> GAGEMRDRIESMFLESWRDYSKHGWGYDVYGPIEHTSHNMPRGNQPLGWIIVDSVDTLMLMYNSSTLYKSEFEAEIQRSEHWINDVLDFDIDAEVNVFETTIRMLGGLLSAYHLSDVLEVGNKTVYLNKAIDLGDRLALAFLSTQTGIPYSSINLHSGQAVKNHADGGASSTAEFTTLQMEFKYLAYLTGNRTYWELVERVYEPLYKNNDLLNTYDGLVPIYTFPDTGKFGASTIRFGSRGDSFYEYLLKQYLLTHETLYYDLYRKSMEGMKKHLLAQSKPSSLWYIGEREQGLHGQLSPKMDHLVCFMGGLLASGSTEGLSIHEARRRPFFSKSDWDLAKG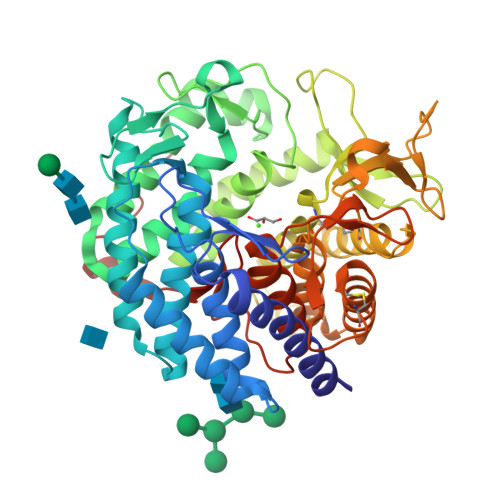ITDTCYQMYKQSSSGLAPEIVVFNDGNIKQDGWWRSSVGDFFVKPLDRHNLQRPETVESIMFMYHLSHDHKYREWGAEIATSFFENTCVDCNDPKLRRFTSLSDCITLPTKKSNNMESFWLAETLKYLYILFLDEFDLTKVVFNTEAHPFPVLDEEILKSQSLTTGWSL> VANPEHYIKHPLQNRWALWFFKNDKSKTWQANLRLISKFDTVEDFWALYNHIQLSSNLMPGCDYSLFKDGIEPMWEDEKNKRGGRWLITLNKQQRRSDLDRFWLETLLCLIGESFDDYSD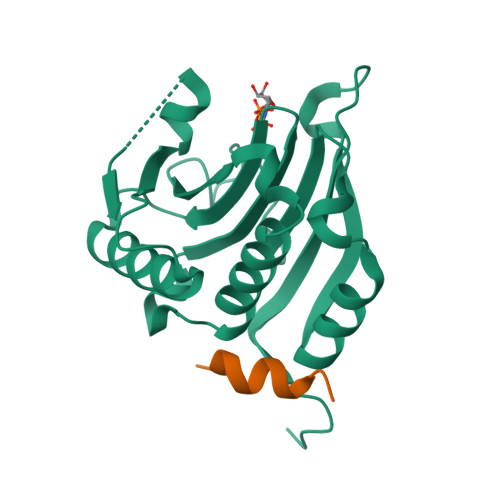DVCGAVVNVRAKGDKIAIWTTECENRDAVTHIGRVYKERLGLPPKIVIGYQSHADTATKSGSTTKNRFVV;> RIIYDRKFLMECRN> PGSVVELLGKSYPQDDHSNLTRKVLTRVGRNLHNQQHHPLWLIKERVKEHFYKQYVGRFGTPLFSVYDNLSPVVTTWQNFDSLLIPADHPSRKKGDNYYLNRTHMLRAHTSAHQWDLLHAGLDAFLVVGDVYRRDQIDSQHYPIFHQLEAVRLFSKHELFAGIKDGESLQLFEQSSRSAHKQETHTMEAVKLVEFDLKQTLTRLMAHLFGDELEIRWVDCYFPFTHPSFEMEINFHGEWLEVLGCGVMEQQLVNSAGAQDRIGWAFGLGLERLAMILYYIPDIRLFWCEDERFLKQFCVSNINQKVKFQPLSKYPAVINDISFWLPSENYAENDFYDLVRTIGGDLVEKVDLIDKFVHPKTHKTSHCYRITYRHMERTLSQREVRHIHQALQEAAVQLLGVEGRF

Mutations in the mitochondrial aminoacyl‐tRNA synthetases (mtaaRSs) can cause profound clinical presentations, and have manifested as diseases with very selective tissue specificity. Among the recently reported pathogenic variants are point mutations in FARS2 gene, encoding the human mitochondrial PheRS. Patient symptoms range from spastic paraplegia to fatal infantile Alpers encephalopathy. How clinical manifestations of these mutations relate to the changes in three‐dimensional structures and kinetic characteristics remains unclear, although impaired aminoacylation has been proposed as possible etiology of diseases.

Here, we report four crystal structures of HsmtPheRS mutants, and extensive MD simulations for wild‐type and nine mutants to reveal the structural changes on dynamic trajectories of HsmtPheRS. Using steady‐state kinetic measurements of phenylalanine activation and tRNAPhe aminoacylation, we gained insight into the structural and kinetic effects of mitochondrial disease‐related mutations in FARS2 gene.V. vulnificus Prx3 (VvPrx3) belongs to the 1-Cys class of Prxs, with one conserved catalytic cysteine (Cys48), and has been shown to be involved in pathogenicity in a mouse model. Cys48 is the CP residue that is crucial for the function of the protein. All three crystal structures of VvPrx3 revealed a protomer exhibiting a compact and spherical structure without a C-terminal extension region, similar to the previously reported 1-Cys Prx AhpE from Mycobacterium tuberculosis (Li et al., 2005). All three crystal structures of VvPrx3 [reduced Prx3 (C48D/C73S), oxidized Prx3 (C73S) and H2O2-bound Prx3 (C48D/C73S)] showed a similar dimeric assembly in the crystals characterized by an A-type dimeric interface, similar to that in AhpE from M. tuberculosis (Li et al., 2005).

To examine the interactions between VvPrx3 and peroxides, the H2O2-bound Prx3 (C48D/C73S) structure was determined at 1.9 Å resolution. A high concentration (500 µM) of H2O2 was incubated with crystals of reduced Prx3 (C48D/C73S), which changed the space group and unit-cell parameters. The H2O2 binding site is fully accessible from the solvent since it is exposed to the external medium. The structure is analogous to that of the H2O2-bound archaeal 2-Cys Prx thio­redoxin peroxidase from Aeropyrum pernix K1, in which the corresponding cysteine residue was overoxidized and shares the H2O2 binding site. Thus, it is likely that substrate binding near CP is important in the rapid catalysis of VvPrx3. In Prx structures only one O atom of H2O2 near Cys48 (or Asp48 in our structure) makes further interactions with VvPrx3, while the other O atom makess no interaction with H2O2-bound Prx3 (C48D/C73S).

>[12x]MIAQGQTLPNATLSQLTKEGMVHHPVLELFAGKKVVLFAVPGAFTPTDSEAHLPGYIVLADQLKAKGVDLIASVSVNDAFVMKAWGEAQNAEEILMLADGDASFTKALGLEMDTAGFGGLRSQRYAMIIDNGVVTTLNVEAPKSFEVSNAETILAALEHHHHHH>MGHHHHHHSGENLYFQSGGMVAPTSNPGVPDELDGVPAVVDCDVHAVLPSPHSLIPYLDEYWADQLVAQLAPTYEPNYHPRGSAIAQHSDASVDENGRAATTAENLVKDVFADGFTDFAVVNCLYGVQQIHQPRREMAHARALNHWIANEWLDKDDRLRASIVVPQGSPRAAAEEIDFWSGDKRFVQVLLLGQSELLYGREINWPIWEAAEAAGLPVTLHIGGVFRQAPTSVGWPASHLEWYVGQQSNIEAQLNSIISEGILQKFPKTKILLSELGFNWLPPFMWKFDKLWKSYRPDIPWVQESPLELIREHVRVTTSPSDGAEEAGRLDSIVDRLGSDRMLVYSSDYPHKHHSGPRDIENGTHSPELLDRIYRRNAFDLYNLVVPSPGKVG[2x];>[2x]MTIIEHGSLGTLPAPSVTTGIVDADIHPVPQDGALEPYLDDRWKKHIREYGVRTTTGLQFISEYPQMYGGAMRADAWPESGYPGSDRELLRTQLLDKHNIQLGVLQCLAPGGQTLNPAGQALNQELAAALCRATNDWQLEHLVYPDPRMRAAIPVTFETPDYAVAEIERVGADPGVVAVLGTSKTLEPLGSRKYWPIYEASVAQNLPIQFHLSQGGGHANTGTGWTSYHTEYHTGHVQSFQSQLLSLVLSGTFDRFPTLKVMFVEGNVAHFAPLIQRMDYTWETLRGELPDLQRKPSEYIRDHIWASTQPIDEPEKPEHLAELLEEFCGDNVVFATDYPHFDFDDPETAFPRSFPVDLRDKILRGNGMRFFGVTNQAD

Here we report that the 2-aminoisobutyric acid hydroxylase from Rhodococcus wratislaviensis, AibH1H2, requires manganese to functionalize a strong, aliphatic C–H bond (BDE = 100 kcal/mol). Structural and spectroscopic studies of this enzyme reveal a redox-active, heterobimetallic manganese–iron active site at the locus of O2 activation and substrate coordination. Metabolism of 2-aminoisobutyric acid (AIB) in Rhodococcus wratislaviensis proceeds via the initial, selective hydroxylation of the pro-(R) methyl group by the monooxygenase AibH1H2 to furnish α-methyl-d-serine (d-MeSer). Previously, recombinant expression of AibH1H2 in Escherichia coli enabled its structural characterization and revealed distinct mono- and dinuclear metal binding sites housed within the AibH1 and AibH2 protein subunits, respectively.

Collectively, these results indicated that the incorporation of two manganese ions and one iron ion afforded the most active form of AibH1H2. To determine the locations of these metal ions, crystallographic studies were performed on active preparations (entry 6) of AibH1H2. The unique locations of metal ions were determined by analysis of the anomalous X-ray dispersion collected at either the Mn K-edge or an anomalous isomorphous difference map stemming from diffraction data collected above and below the Fe K-edge. Two AibH1H2 heterodimers are found in the asymmetric unit. Both AibH1 subunits display strong anomalous scattering at the Mn K-edge above background levels and lack observable density at the Fe K-edge difference map at Site 0, supporting exclusive Mn binding at these sites. In contrast, the dinuclear sites in AibH2 appear in two distinct metalated forms. View 1 of AibH2 contains a dimanganese site with a fully occupied Site 1 metal and a partially occupied (∼60%) Site 2 metal. View 2 of AibH2 contains two fully occupied sites with predominant Fe occupancy in Site 1 and exclusive manganese occupancy in the solvent-exposed Site 2. Since this latter view represents the only location of observable Fe content throughout the structure, we hypothesize that the bimetallic arrangement of View 2 represents the correctly metalated form of AibH1H2 that participates in substrate hydroxylation. In this scenario, Site 1 is the expected and observed position for FeII binding, as the coordination environments of Sites 1 and 2 contain five and three amino-acid-derived ligands, respectively.>MGLAEGLAARMAPHLYIQEPLSAQQLKKLEEHKYSASGRSLVEPPMQVYWNWLVEKVPLWLAPNTITMVGLLLNVLSTLILVCYCPTATEGAPFWTYLLCAIGLFVYQSLDAIDGKQARRTNSSSPLGEMFDHGCDSISIVFVNLGTIAAVRLGTLPGWMFYCCFVGMFMFYCAQWQTYVCGTLKFGIIDVTELQISVTVMFLMTAVCGPELWDYEIPFTGLPMKTIPLLGIIGGTVYSCSNYFRVILSGGVGKNGSTVAGTSVLSPGLHIGLVLLLALMIYKKSTTNLFLQNPCLYTLAFGFVSAKITIKLVIAHMTKSEISLQDTAFIGPGLLFFNQYFNSFIDEYIVLWIAMVISFADLLRYCISVCLQIATHLRISVFRISSNQAAEQVQTQKQKLTD[2x]

In eukaryotes, two highly homologous enzymes, cholinephosphotransferase-1 (CHPT1) and choline/ethanolamine phosphotransferase-1 (CEPT1) catalyze the final step of de novo PC synthesis. CHPT1/CEPT1 joins two substrates, cytidine diphosphate-choline (CDP-choline) and diacylglycerol (DAG), to produce PC, and Mg2+ is required for the reaction. Here we report structures of a CHPT1 from Xenopus laevis (xlCHPT1) determined by cryo-electron microscopy to an overall resolution of ~3.2 Å. xlCHPT1 forms a homodimer, and each protomer has 10 transmembrane helices (TMs). The first 6 TMs carve out a cone-shaped enclosure in the membrane in which the catalysis occurs.

We determined two structures of xlCHPT1 by single-particle cryo-electron microscopy (cryo-EM). The structure of xlCHPT1 in complex with CDP-choline and Mg2+ has an overall resolution of ~3.7 Å, and that of xlCHPT1 in complex with CDP and Mg2+, ~3.2 Å resolution. Density for two Mg2+ are prominent in both cryo-EM maps, and the Mg2+ are coordinated by side chain carboxylates of Asp111, Asp114 from TM2 and Asp132, Asp136 from TM3. The side chain carboxylates of Asp111 and Asp132 interact with both Mg2+ simultaneously, forming two bidentate bridges. We define the Mg2+ that interacts with Asp114 as Mg1 and the other one as Mg2. Densities for CDP or CDP-choline are clearly recognizable, with the cytidine ring coordinated by the side chain of Asn64 and by the backbone nitrogen of Ser124. The diphosphate group in CDP is coordinated by Mg1, the side chain guanidinium group of Arg119, and the side chain hydroxyl group of Tyr34. The two residues do not have direct interactions with Mg2+ or CDP-choline but His133 is ~7 Å away from the β-phosphate of CDP. In both density maps, there are tubular shaped non-protein densities resembling two acyl chains at the entrance of the slit, suggesting that the slit is wide enough to accommodate two acyl chains.> GHMLDCKAVALKWVHQFRIPGGDNCNFYCSYDSLYQQFNLWKKNDACQGADGFSTAIPKIQEAPCSDCPGSKTCICSVQATAWRVRNGKWFDGQQWFDCDVKPYTERVLGRRWYDESEADKDIYVGYYSRGFISNDNVHCGSQ

The Dothideomycete Leptosphaeria maculans, causal agent of oilseed rape stem canker or blackleg disease, is one of the fungal pathogens in which suppression of ETI by the presence of an AVR gene has been demonstrated. Among them, AvrLm4-7 suppresses Rlm3-mediated resistance triggered by AvrLm3 and Rlm9-mediated resistance triggered by AvrLm5-9. Surprisingly, despite low sequence similarity, AvrLm5-9 and AvrLm3 are structural analogues of AvrLm4-7, sharing an anti-parallel β-sheet covered by α-helices. Structure-informed sequence database searches identified a larger number of putative structural analogues among L. maculans effector candidates, including the AVR effector AvrLmS-Lep2, all produced during the early stages of oilseed rape infection, as well as among effector candidates from other phytopathogenic fungi. These structural analogues are named LARS (for Leptosphaeria AviRulence and Suppressing) effectors.

A small secreted protein with 37% amino acid sequence identity with AvrLm3 was identified from F. fulva. The analysis of the anomalous signal revealed the presence of two Zn-clusters in the structure that resemble those of the Ni-ions in AvrLm5-9. One Zn-cluster is bound near the N- and C-termini and involves histidines from the native protein and from the linker peptide and side chains from a crystal neighbor. Strands β1 and β2 are connected by a peptide composed of a helical turn and a short helix surrounded by irregular peptides. The long connection between strands β3 and β4 contains a β-hairpin, a short helix and some irregular peptide stretches. The sequence alignment and structure superposition show conservation of all 10 cysteines, suggesting both proteins form an identical set of disulfide bridges. The sequence similarities between AvrLm5-9, AvrLm4-7 and Ecp11-1/AvrLm3 are relatively weak (between 18 and 28%). Nevertheless, the 3D structures of all these effectors are strongly related: AvrLm5-9 and Ecp11-1/AvrLm3 share the same fold with AvrLm4-7, which displays suppressive interactions with AvrLm5-9 and AvrLm3. All three effectors have a disulfide bridge that connects the N- and C-termini, and also at least one disulfide bridge that links the helical connection between β1-β2 and strand β3.Since ENPP1 is part of the highly conserved nucleotide pyrophosphatase/phosphodiesterase (NPP) protein family, we investigated the evolutionary conservation of the analogous histidine residue and its requirement for cGAMP degradation. Two zinc ions are required for NPP’s catalytic activity, with Zn1 being particularly important for stabilizing the leaving group, whereas Zn2 activates the threonine nucleophile. We found that Xac NPP not only degrades cyclic dinucleotides but also prefers 2′-5′–linked over 3′-5′–linked cyclic dinucleotides. Furthermore, the conserved histidine is required for degrading the 2′-5′ but not 3′-5′ phosphodiester linkage.

As mouse ENPP1 is technically challenging to crystallize, we took advantage of the conservation between Xac NPP and mouse ENPP1 to solve the cocrystal structure of Xac NPP in complex with cGAMP. To prevent cGAMP hydrolysis, we mutated the catalytic threonine to alanine (Xac NPP T90A), crystalized it with cGAMP, and obtained a 1.9 Å crystal structure. Similar to the previous mouse ENPP1 T238A structure, we found a linear 3′-5′–linked pApG intermediate bound to NPP instead of intact cGAMP. In the previous structure, the guanine ring was within stacking distance of the conserved histidine (∼4.5 Å). However, the guanine ring in our structure is ∼8 Å away from the histidine and rotated 140° from the previous structure. This discrepancy suggests that the guanine ring is flexible and mobile, which explains why mutating the guanosine-adjacent site did not disrupt cGAMP hydrolysis. Using cGAMP as a competitive inhibitor of the ENPP1-ATP reaction, we determined that ENPP1WT and ENPP1H362A have very similar Ki values, demonstrating that ENPP1H362A binds cGAMP equally well as ENPP1WT. Together, our structural and biochemical data demonstrate that H362 is not necessary for binding cGAMP.

>MIDRRFGVAAAALALLAACSSPPSARSAPTQLPTAAPGTASASTPHALLLISIDGLRADMLDRGITPNLSHLAREGVRARWMAPSYPSLAFPNHYTLVTGLRPDHHGIVHNSMRDPTLGGFWLSKSEAVGDARWWGGEPVWVGVENTGQHAATWSWPGSEAAIKGVRPSQWRHYQKGVRLDTRVDAVRGWLATDGAQRNRLVTLYFEHVDEAGHDHGPESRQYADAVRAVDAAIGRLLAGMQRDGTRARTNIIVVSDHGMAEVAPGHAISVEDIAPPQIATAITDGQVIGFEPLPGQQAAAEASVLGAHDHYDCWRKAELPARWQYGSHPRIPSLVCQMHEGWDALFPDKLAKRAQRGTRGSHGYDPALPSMRAVFLAQGPDLAQGKTLPGFDNVDVYALMSRLLGIPAAPNDGNPATLLPALRMPP[6x]>MHADTATRQHWMSVLAHSQPAELAARLNALNITADYEVIRAAETGLVQIQARMGGTGERFFAGDATLTRA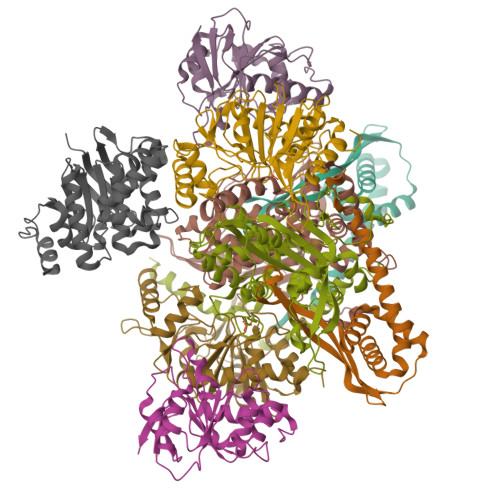AVRLTDGTLGYSWVQGRDKQHAERCALIDALMQQSRHFQNLSETLIAPLDADRMARIAARQAEVNASRVDFFTMVRGDNA[2x];>[2x]MTLETAFMLPVQDAQHSFRRLLKAMSEPGVIVALHQLKRGWQPLNIATTSVLLTLADNDTPVWLSTPLNNDIVNQSLRFHTNAPLVSQPEQATFAVTDEAISSEQLNALSTGTAVAPEAGATLILQVASLSGGRMLRLTGAGIAEERMIAPRLPECILHELTERPHPFPLGIDLILTCGERLLAIPRTTHVEVC;>MYVAVKGGEKAIDAAHALQESRRRGDTDLPELSVAQIEQQLNLAVDRVMTEGGIADRELAALALKQASGDNVEAIFLLRAYRTTLAKLAVSEPLDTTGMRLERRISAVYKDIPGGQLLGPTYDYTHRLLDFTLLANGEAPTLTTADSEQQPSPHVFSLLARQGLAKFEEDSGAQPDDITRTPPVYPCSRSSRLQQLMRGDEGYLLALAYSTQRGYGRNHPFAGEIRSGYIDVSIVPEELGFAVNVGELLMTECEMVNGFIDPPGEPPHFTRGYGLVFGMSERKAMAMALVDRALQAPEYGEHATGPAQDEEFVLAHADNVEVAGFVSHLKLPHYVDFQAELELLKRLQQEQNHG[2x];>MANLSGYNFAYLDEQTKRMIRRAILKAVAIPGYQVPFGGREMPMPYGWGTGGIQLTASVIGESDVLKVIDQGADDTTNAVSIRNFFKRVTGVNTTERTDDATVIQTRHRIPETPLTEDQIIIFQVPIPEPLRFIEPRETETRTMHALEEYGVMQVKLYEDIARFGHIATTYAYPVKVNGRYVMDPSPIPKFDNPKMDMMPALQLFGAGREKRIYAVPPFTRVESLDFDDHPFTVQQWDEPCAICGSTHSYLDEVVLDDAGNRMFVCSDTDYCRQQSEAKNQ[2x];> MNQPLLSVNNLTHLYAPGKGFSDVSFDLWPGEVLGIVGESGSGKTTLLKSISARLTPQQGEIHYENRSLYAMSEADRRRLLRTEWGVVHQHPLDGLRRQVSAGGNIGERLMATGARHYGDIRATAQKWLEEVEIPANRIDDLPTTFSGGMQQRLQIARNLVTHPKLVFMDEPTGGLDVSVQARLLDLLRGLVVELNLAVVIVTHDLGAARLLADRLLVMKQGQVVESGLTDRVLDDPHHPYTQLLVSSVLQNHHHHHH>ARASVLSGGELDKWEKIRLRPGGKKQYKLKHIVWASRELERFAVNPGLLETSEGCRQILGQLQPSLQTG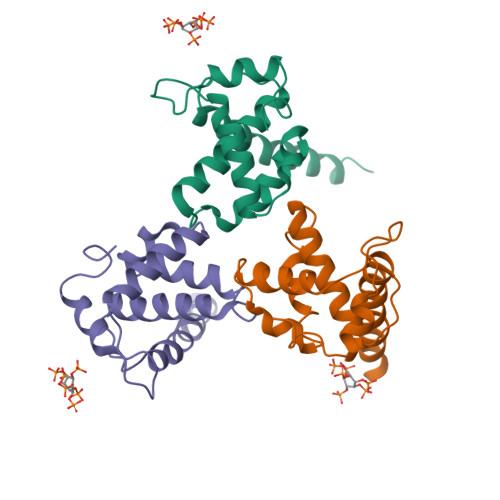SEELRSLYNTIAVLYCVHQRIDVKDTKEALDKIEEEQNKSKKKAQQAAADTG[12x]> GSHMTSSANEGSHMTSSANEDMPVERILEAELAVEPKTETYVEANMGLNPSSPNDPVTNICQAADKQLFTLVEWA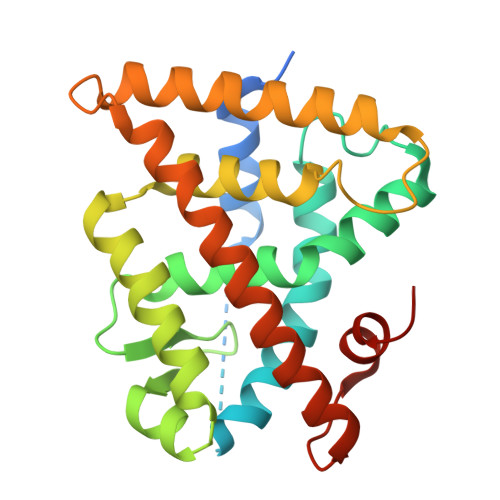KRIPHFSELPLDDQVILLRAGWNELLIASFSHRSIAVKDGILLATGLHVHRNSAHSAGVGAIFDRVLTELVSKMRDMQMDKTELGCLRAIVLFNPDSKGLSNPAEVEALREKVYASLEAYCKHKYPEQPGRFAKLLLRLPALRSIGLKCLEHLFFFKLIGDTPIDTFLMEMLEAPHQMT In Gram-positive bacteria, nitrogen homeostasis is controlled by an operon encoding glutamine synthetase (GS), a dodecameric machine that assimilates ammonium into glutamine, and the GlnR repressor. GlnR detects nitrogen excess indirectly by binding glutamine-feedback-inhibited-GS (FBI-GS), which activates its transcription-repression function. GS generates glutamine from glutamate, ATP, and ammonium by a mechanism that involves the initial phosphorylation of the γ-carboxyl group of glutamate by ATP and the subsequent incorporation of ammonium. The structures show FBI-GS binds the GlnR C-terminal domain within its active-site cavity, juxtaposing two GlnR monomers to form a DNA-binding-competent GlnR dimer.

To ascertain if this is a conserved mechanism among FBI-GS-GlnR complexes and to elucidate, in detail, the molecular mechanism by which low G + C Gram-positive FBI-GS proteins bind GlnR, we utilized single-particle cryo-electron microscopy (cryo-EM) and solved high-resolution structures of the Bs (1.96 Å), Lm (2.61 Å), Pp (2.07-2.28 Å), and Sa (2.15 Å) FBI-GS-GlnR C-tail complexes. Notably, the Bs and Lm GS proteins in the complexes were all tetradecameric, while the Pp GS in the complex formed 10% tetradecamers and 90% dodecamers and the GS in the Sa FBI-GS-GlnR structure was all dodecameric. D Density for GlnR peptide and contacts with GS in the Sa FBI-GS-GlnR complex (map contoured at 0.15 σ). Peptide density was evident for 8-10 residues of the GlnR C-tails from Pp (IQGELSRF), Sa (PINRGDLSRF), and Bs (FRQGDMSRF), and 5 GlnR C-terminal residues (QLPRF), in the Lm complex. These GlnR C-tails all form a distorted helix and bind within the GS active sites. In the FBI-GS-GlnR structures, each GS pore binds two closely juxtaposed but non-interacting GlnR C-tails as each pore contains two active sites, one from each ring. The GlnR C-tails in all but the Lm structure contains a glycine at the N-terminal region of the bound peptide (XG(E/D)XSRF). This glycine binds proximal to the E flap, allowing its amide nitrogen to H bond with the carbonyl oxygen of the GS glycine residue in the E flap. The GlnR arginine of this motif makes contact with residues on α15´´ and stacks with the side chain of the aromatic residue in the GS D50´ loop in the Pp, Sa, and Bs structures. The flexible connection between these domains would thus be minimally comprised of ~30 residues (calculated as the number of residues between the first and last residues visible in the Sa GS-GlnR and Sa GlnR structures; the Bs and Lm disordered linkers are >40 residues), which if fully extended could span >90 Å.

>GSHMPKRTFTKEDIRKFAEEENVRYLRLQFTDILGTIKNVEVPVSQLEKVLDNEMMFDGSSIEGFVRIEESDMYLHPDLDTWVIFPWTAGQGKVARLICDVYKTDGTPFEGDPRANLKRVLKEMEDLGFTDFNLGPEPEFFLFKLDEKGEPTLELNDDGGYFDLAPTDLGENCRRDIVLELEDMGFDIEASHHEVAPGQHEIDFKYADAVTACDNIQTFKLVVKTIARKHNLHATFMPKPLFGVNGSGMHFNVSLFKGKENAFFDPNTEMGLTETAYQFTAGVLKNARGFTAVCNPLVNSYKRLVPGYEAPCYIAWSGKNRSPLIRVPSSRGLSTRIEVRSVDPAANPYMALAAILEAGLDGIKNKLKVPEPVNQNIYEMNREEREAVGIQDLPSTLYTALKAMRENEVIKKALGNHIYNQFINSKSIEWDYYRTQVSEWERDQYMKQY[12x];>[12x]PINRGDLSRFI>GSHMQSDSAVLQWANQAAIAAFTYNFVNYRDELQASSGFFTAEGWDQFLGALEQSNNLDAVKAKKLVVSAVATRAPIILQKGVLNGRYSWRV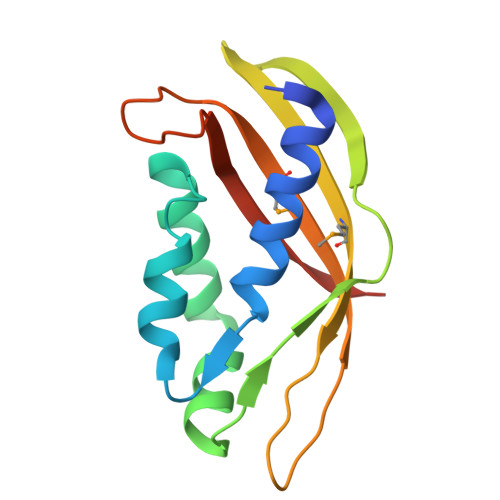QMPILVTYQSASEFTQQNNVVTMLITRVSTLNSPRGIGISQFVVGPASGGVS[4x]>MAELACFVSFSLTEDKVVWYPINKKAVQTMLCAKVEKDQRSNYYDTILYGVAPPPEFRNRFKTNERYGLDYESDQYTELVNLLADTLNMVSMPTEKFQFDIVKTVVQVRHLENLLCRIKDVNDILNANVKLRVKAVMIACNLVNETETTPLTESNDIVYQDSYFTITKLDYSNHKLLPLMADEYKITINTKTDIPDRNQTAFAAYIRYNFNKFAAISHGKRHWRLVLHSQLMSHAERLDRKIKSDKKHGRQFSYDDGDMAFVHPGWKTCIGQLCGGT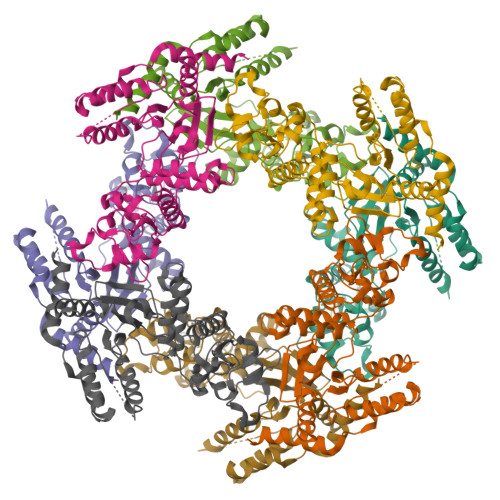TFEVAKTSLYSIKPSKTVRTATNKIESDLISMVGN[2x]>[5x]MSGMRVYLGADHAGYELKQRIIEHLKQTGHEPIDCGALRYDADDDYPAFCIAAATRTVADPGSLGIVLGGSGNGEQIAANKVPGARCALAWSVQTAALAREHNNAQLI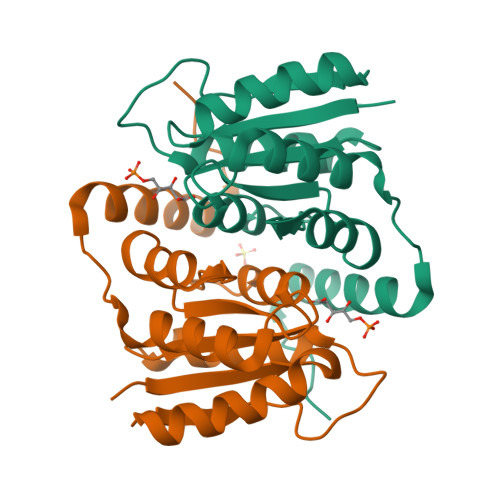GIGGRMHTVAEALAIVDAFVTTPWSKAQRHQRRIDILAEYERTHEAPPVPGAPA(E,2S)-2-[(1R,3aS,4E,7aR)-7a-methyl-4-[2-[(3R,5R)-4-methylidene-3,5-bis(oxidanyl)cyclohexylidene]ethylidene]-2,3,3a,5,6,7-hexahydro-1H-inden-1-yl]oct-6-en-4-yn-3-one 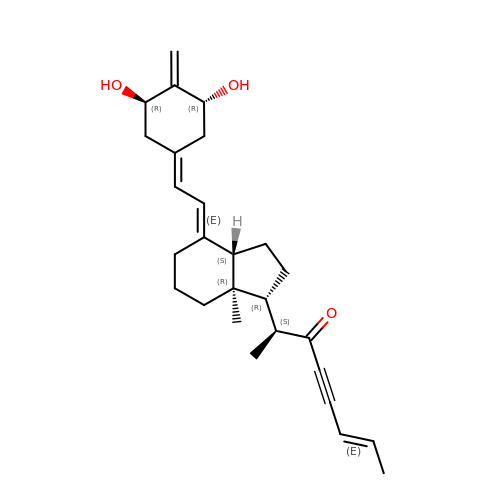| C27 H36 O3 | LQJPGHNFADIMOG-QHQWRQFTSA-N>[2x]MWRIELKHAVNWELKMKFFVLPELPTPDVVESGVWRRAIVLDGRAVAVMAYPESERTIVVEGNFENREWEAVRRKLVEYLGLQNPEELYRFMDGDEKLRMLKNRFYGFGRAGLMSMSVFEGIAKAIIQQQISFVVAEKLAAKIVGRFGDEVEWNGLKFYGFPTQEAILKAGVEGLRECGLSRRKAELIVEIAKEEN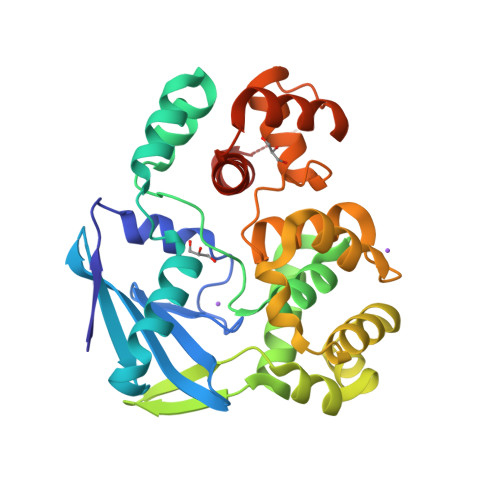LEELKEWGEEEAYEYLTSFKGIGRWTAELVLSMALGKNVFPADDLGVRRAVSRLYFNGEIQSAEKVREIARERFGRFARDILFYLFLYDRFFSKKTELV> MEFSGRKWRKLRLAGDQRNASYPHCLQFYLQPPSENISLIEFENLAIDRVKLLKSVENLGVSYVKGTEQYQSKLESELRKLKFSYRENLEDEYEPRRRDHISHFILRLAYCQSEELRRWFIQQEMDLLRFRFSILPKDKIQDFLKDSQLQFEAISDEEKTLREQEIVASSPSLSGLKLGFESIYKIPFADALDLFRGRKVYLEDGFAYVPLKDIVAIILNEFRAKLSKALALTA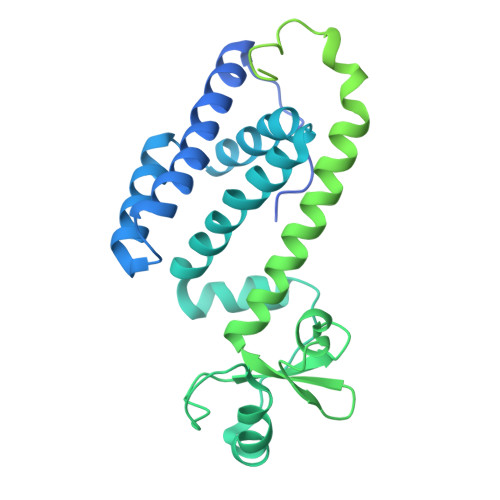RSLPAVQSDERLQPLLNHLSHSYTGQDYSTQGNVGKISLDQIDLLSTKSFPPCMRQLHKALRENHHLRHGGRMQYGLFLKGIGLTLEQALQFWKQEFIKGKMDPDKFDKGYSYNIRHSFGKEGKRTDYTPFSCLKIILSNPPSQGDYHGCPFRHSDPELLKQKLQSYKISPGGISQILDLVKGTHYQVACQKYFEMIHNVDDCGFSLNHPNQFFCESQRILNGGKDIKKEPIQPETPQPKPSVQKTKDASSALASLNSSLEMDMEGLEDYFSEDS>[2x]SNAMNEPIILRYFPVLGRAQALRHALADAELAFRDLRIPLEQWSQHKDSDAGGPYGSLPTLRWHGVEVAETIAIASFLARSLGHYEGRDNGEIARLEAVVSLCYTEVSLQIAQLLWLDLFNP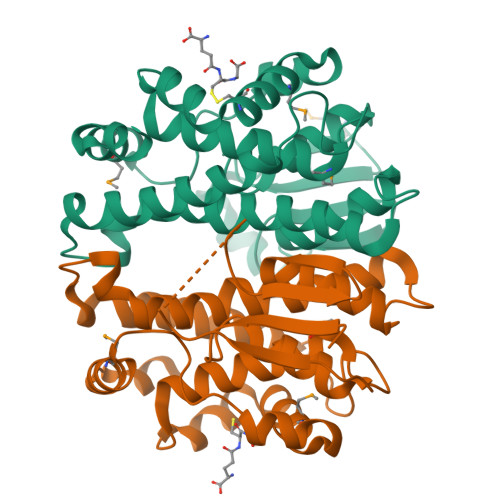GVDLAAAVPLQFGRLVARLTRLEAHTPEAGWFGGERPVMADYFAAEAIEALRYLLGREHDDALRTRLPHLCALARRMAQRPALAQAWSTRPQTFTAHPDEAAMLERLRALPLAATIGASME3-disulfanylpropanoic 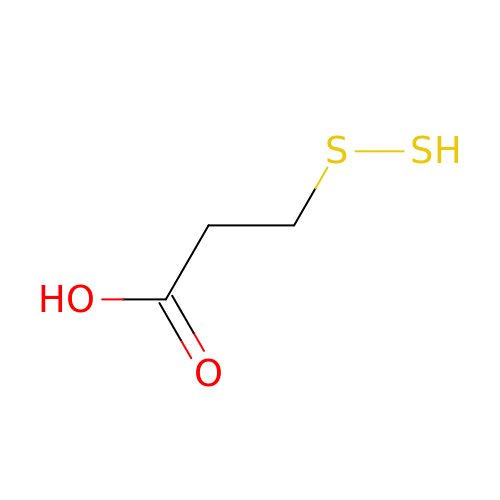acid | C3 H6 O2 S2 | CXXDUKKBFUFJDF-UHFFFAOYSA-N>LTCVTSKSIFGITTENCPDGQNLCFKRWQYISPRMYDFTRGCAATCPKAEYRDVINCCGTDKCNK[3x]

The three-finger toxin (3FT) family is widely represented as structural motif, mainly in the Elapidae snake venoms, supporting various biological functions. This fold is characterized by three adjacent loops rich in β-pleated sheets emerging from a small globular core containing four invariant disulfide bridges. Despite high primary structure identity, often greater than 55%, muscarinic and adrenergic toxins exhibit distinct pharmacological profiles and clear functional differences. “Loop grafting” has been used to construct seven chimeric toxins to dissect how the affinity, selectivity and functionality for the muscarinic and adrenergic receptors depend on shuffling loops between various toxins.

Three chimeras were obtained by substituting loops of the MT7 toxin with the corresponding loop from the MT1. These chimeras were named MT7-1/1, MT7-1/2 and MT7-1/3, numbered for the respective grafted MT1 loop. Loop 1 of each of the three molecules in the asymmetric unit of MT7-1/1 superimposes precisely on that of loop 1 of MT1. The loop separates from loops 2 and 3 as it does in MT1 but to a greater extent. The grafted loop 1 of chimera MT7-1/1 preserves its structure as in MT1 but does not adopt the same relationship with loop 2 as in MT1 nor keep the relationship found between loop 1 and loop 2 of MT7. Thus a new toxin with novel properties is created by the grafting. If MT7 is compared to chimera MT7-1/1, least-squares gives an rmsd of 3.13±0.02 Å while by SSM gives 1.4 Å. On hM1 receptor, substitutions of MT7 loops 1 and 3 by those of MT1 (chimeras MT7-1/1 and MT7-1/3) have no significant impact on the toxin affinity, suggesting that the seven modifications associated with each of these substitutions were not involved in the high affinity of the MT7-hM1 interaction. Notably, a two orders of magnitude increase in affinity for the α1A-adrenoceptor is achieved for chimeras MT7-1/1 and MT7-1/3 by the grafting of loop 1 or 3. These toxins are characterized by an affinity close to that of MT1 for the α1A-adrenoceptor.N-[3-[(4S)-2-azanyl-4-methyl-5,6-dihydro-1,3-thiazin-4-yl]-4-fluoranyl-phenyl]-5-chloranyl-pyridine-2-carboxamide | C17 H16 Cl F N4 O S | 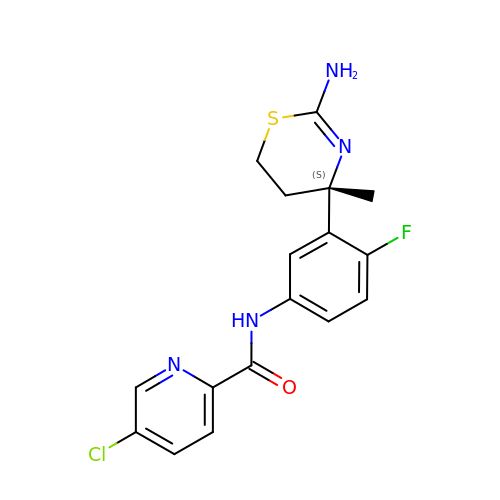VVZZZUNCWSTIOI-KRWDZBQOSA-N> MSFRKRGEILNDRGSGLRGPLLRGPPRTSSTPLRTGNRRAPGNVPLSDTTARLKKLNIADESKTKMGLDSSHVGVRPSPATSQPTTSTGSADLDSILGHMGLPLGNSVLVEEQSTTEFHSILGKLFAAQGIVHNRISDSSADKTRNGDTHVIVLSLNQMFAKELPGIYKGSRKQMKKNLISEEESKVTVQNLNETQRSTPSRYKDLKIAWKYKLADEKRLGSPDRDDIQQNSEYKDYNHQFDITTRLMPAPIASELTFIAPTQPVSTILSQIEQTIKRNDKKLIRIVIPSLLHPAMYPPKMFESSEIIGLMHGVRSLVKKYYERVVLFASISIDIITPPLLVLLRNMFDSVINLEPFNQEMTEFLERVYKSQPGKIQHGLVHILKLPVFTDRGEMRVLKSEWAF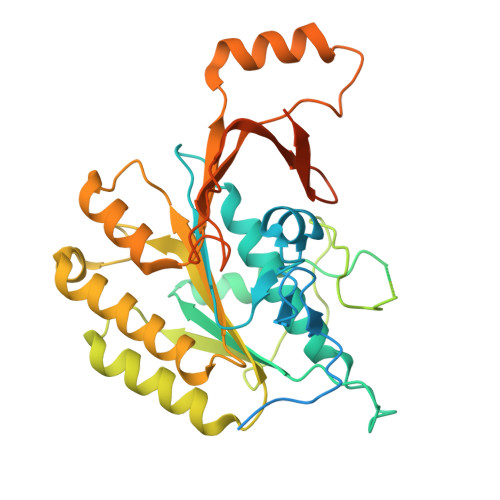KNGRKKFEIEQWGIPVDDAEGSAASEQSHSHSHSDEISHNIPAKKTKISLDY> MIDIENEITEFFNKMRDTLPAKDSKWLNPSCMFGGTM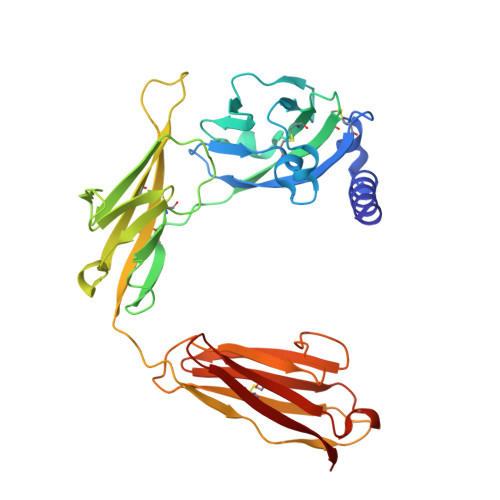NDMAALGEPFSAKCPPIEDSLLSHRYNDKDNVVNWEKIGKTRRPLNRRVKNGDLWIANYTSNDSHRRYLCTVTTKNGDCVQGIVRSHIRKPPSCIPETYELGTHDKYGIDLYCGILYAKHYNNITWYKNNQELIIDGTKYSQSGQNLIIHNPELEDSGRYDCYVHYDDVRIKNDIVVSRCKILTVIPSQDHRFKLILDPKINVTIGEPANITCTAVSTSLLVDDVLIDWENPSGWIIGLDFGVYSILTSSGGITEATLYFENVTEEYIGNTYTCRGHNYYFDKTLTTTVVLE>[2x]SMSPNGNLIRMLVLFFLESELHEHAAYLVDSLWESSQELLKDWECMTELLLEEPVQGEEAMSDRQESALIELMVCTIRQAAEAHPPVGRGTGKRVLTAKERKTQIDDRNKLTEHFIITLPMLLSKYSADAEKVANLLQIPQYFDLEIYSTG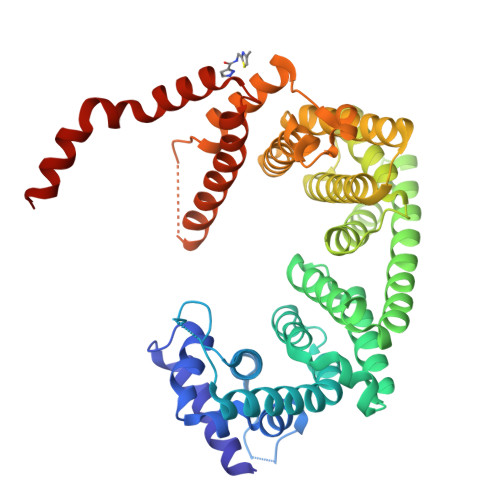RMEKHLDALLKQIKFVVEKHVESDVLEACSKTYSILCSEEYTIQNRVDIARSQLIDEFVDRFNHSVEDLLQEGEEADDDDIYNVLSTLKRLTSFHNAHDLTKWDLFGNCYRLLKTGIEHGAMPEQIVVQALQCSHYSILWQLVKITDGSPSKEDLLVLRKTVKSFLAVCQQCLSNVNTPVKEQAFMLLCDLLMIFSHQLMTGGREGLQPLVFNPDTGLQSELLSFVMDHVFIDQDEENQSMEGDEEDEANKIEALHKRRNLLAAFSKLIIYDIVDMHAAADIFKHYMKYYNDYGDIIKETLSKTRQID>[2x]MKTIIINGVQFNTDEDTTILKFARDNNIDISALCFLNNCNNDINKCEICTVEVEGTGLVTACDTLIEDGMIINTNSDAVNEKIKSRISQLLDIHEFKCGPCNRRENCEFLKLVIKYKARASKPFLPKDKTEYVDERSKSLTVDRTKCLLCGRCVNACGKNTETYAMKFLNKNGKTIIGAEDEKCFDDTNCLLCGQCIIACPVAALSEKSHMDRVKNALNAPEKHVIVAMAPSVRASIGELFNMGFGVDVTGKIYTALRQLGFDKIFDINFGADMTIMEEATELVQRIENNGPFPMFTSCCPGWVRQAENYYPELLNNLSSAKSPQQIFGTASKTYYPSISGLDPKNVFTVTVMPCTSKKFEADRPQMEKDGLRDIDAVITTRELAKMIKDAKIPFAKLEDSEADPAMGEYSGAGAIFGATGGVMEAALRSAKDFAENAELE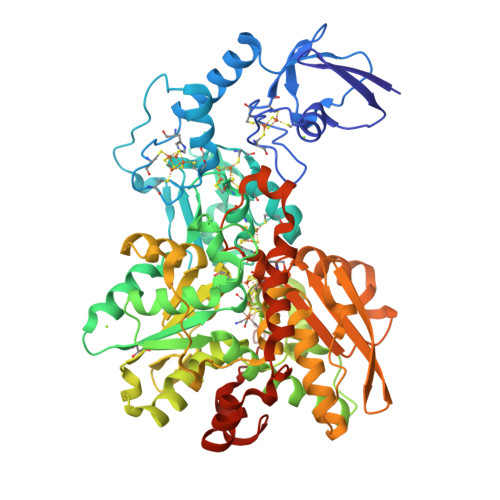DIEYKQVRGLNGIKEAEVEINNNKYNVAVINGASNLFKFMKSGMINEKQYHFIEVMACHGGCVNGGGQPHVNPKDLEKVDIKKVRASVLYNQDEHLSKRKSHENTALVKMYQNYFGKPGEGRAHEILHFKYKKSAWSHPQFEK[1-(3-HYDROXY-2-OXO-1-PHENETHYL-PROPYLCARBAMOYL)2-PHENYL-ETHYL]-CARBAMIC 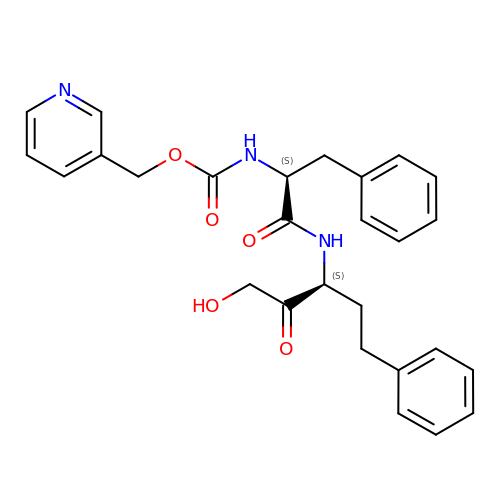ACID PYRIDIN-4-YLMETHYL ESTER | C27 H29 N3 O5 | QCUBCTPTNWPFBC-ZEQRLZLVSA-N>[4x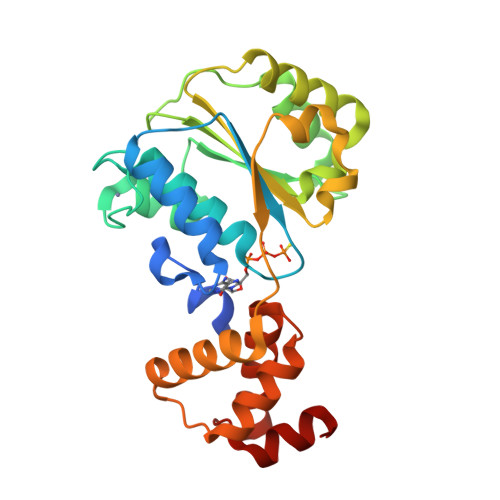]GAHMGGSMSYQVLARKWRPQTFADVVGQEHVLTALANGLSLGRIHHAYLFSGTRGVGKTSIARLLAKGLNCETGITATPCGVCDNCREIEQGRFVDLIEIDAASRTKVEDTRDLLDNVQYAPARGRFKVYLIDEVHMLSRHSFNALLKTLEEPPEHVKFLLATTDPQKLPVTILSRCLQFHLKALDVEQIRHQLEHILNEEHIAHEPRALQLLARAAEGSLRDALSLTDQAIASGDGQVSTQAVSAMLGT> EDICFIAGIGDTNGYGWGIAKELSKRNVKIIFGIWPPVYNIFMKNYKNGKFDNDMIIDKDKKMNILDMLPFDASFDTANDIDEETKNNKRYNMLQNYTIED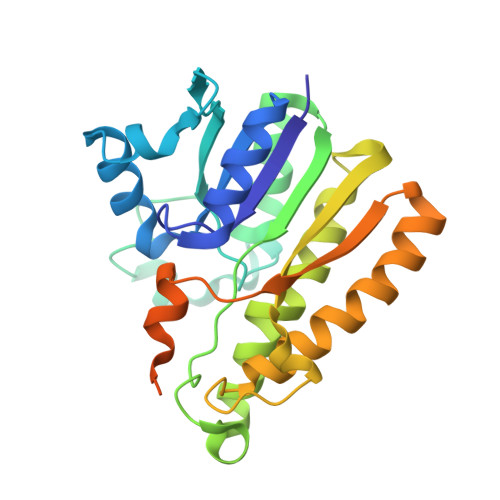VANLIHQKYGKINMLVHSLANAKEVQKDLLNTSRKGYLDALSKSSYSLISLCKYFVNIMKPQSSIISLTYHASQKVVPGYGGGMSSAKAALESDTRVLAYHLGRNYNIRINTISAGPLKSRAATAINKLNNTYENNTNQNKNRNSHDVHNIMNNSGEKEEKKNSASQN>[2x]MGSDKIHHHHHHENLYFQGMSVAHENARRIISDILGKQNIERVWFVGCGGSLTGFWPGKYFLDCEASKLAVGYITSNEFVHATPKALGKNSVVILASQQGNTAETVAAARVAREKGAATIGLVYQPDTPLCEYSDYIIEYQWARYPETVDPAQQKA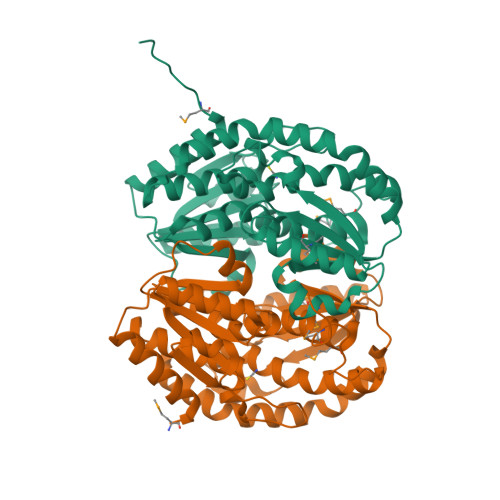AYSLWLALEILAQTEGYAQYDELVSAFGRFSDVVHGAQRQVQEDAQRFAAEWKDEKVVYMMGSGPSFGAAHQESICILLEMQWINSASIHSGEYFHGPFEITEPGTPFILLQSSGRTRPLDDRAIRFIERYQGKLQLIDADKLGIQDLSTDVGEYFCGLLHNCVLDVYNLALATARNHPLTTRRYMWKVEY> GGAU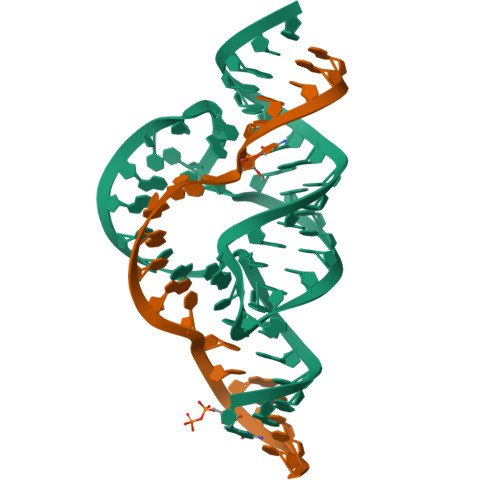GUACUACCAGCUGAUGAGUCCCAAAUAGGACAAAACGCC;> GGCGUCCUGGUAUCCAAUCC> GMTAPVDGSALEARVGHYYQMDNPYLVGREKVREYARAVQDYHPSHWDAAAAADLGYSGVVAPLTFTSTPAMACNRRMFESVVVGYDTYLQTEEVFEQHRPIVAGDELHIDVELTSIRRVAGRDLITVTNTFTDMAGERVHTLHTTVVGITADEISPGTMAAVQKAMMHDVDFSGIGAPGDSYIKT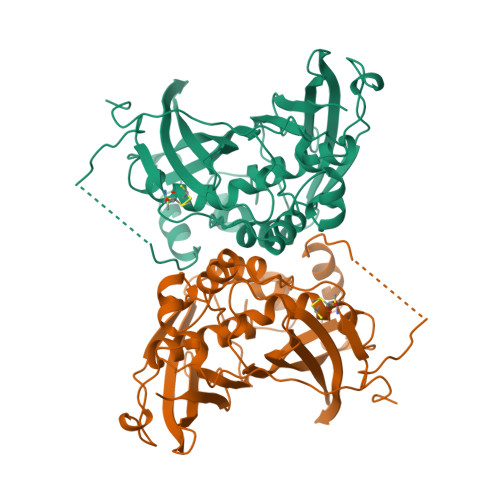VRPAGEVRVAQDTARNPGTPSFDDVKVGDELPVHHTRLSRGDLVNYAGVAGDANPIHWDEEIAKLAGLPDVIAHGMLTMGLGAGFFSAWSGDPGAVTRYAVRLSAPAIVSAAEGADIEFGGKIKSLDPQTRTGIVVVTAKASGKKIFGLATMSVRFS>[2x]MPNIKIFSGSSHQDLSQKIADRLGLELGKVVTKKFSNQETCVEIGESVRGEDVYIVQSGCGEINDNLMELLIMINACKIASASRVTAVIPCFPYARQDKKDKSRAPISAKLVANMLSVAGADHIITMDLHASQIQGFFDIPVDNLYA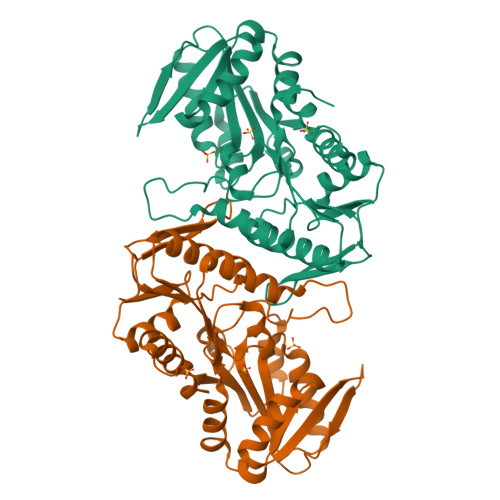EPAVLKWIRENISEWRNCTIVSPDAGGAKRVTSIADRLNVDFALIHKERKKANEVDRMVLVGDVKDRVAILVDDMADTCGTICHAADKLLSAGATRVYAILTHGIFSGPAISRINNACFEAVVVTNTIPQEDKMKHCSKIQVIDISMILAEAIRRTHNGESVSYLFSHVPLLEHHHHHH Here, we demonstrate the determination of the crystal structures of T. brucei GMPR; a protein that, unlike the GMPRs of host animals, possesses a CBS domain. We further show that TbGMPR activity is regulated by purine nucleotide binding to an allosteric regulatory site formed at the cleft between the catalytic and CBS domains of the enzyme. Our kinetic and structural analyses clearly demonstrate that the CBS domain has a pivotal role in the allosteric regulation of the activity and structure of TbGMPR, facilitating the transitions among three conformations: a tetramer, and octamers with relaxed and twisted conformations. A combination of X-ray crystallography and size-exclusion chromatography small-angle X-ray scattering (SEC-SAXS) analysis clearly revealed that TbGMPR can exist as a tetramer or an octamer depending on the nucleotide species that is bound to the CBS domain.

We also determined the structure of TbGMPR C318A with substrate GMP (C318A/GMP) at 1.90-Å resolution and found that C318A/GMP adopted an octameric structure as observed in C318A apo. However, two tetramers in the C318A/GMP octamer were arranged in a twisted position around the fourfold axis compared to C318A apo, and the overall structure of the C318A/GMP octamer was compressed along the fourfold axis. Thus, it appears that GMP induces the transformation of TbGMPR from a “relaxed” (C318A apo) to a “twisted” form (C318A/GMP). Two GMP molecules were observed in each subunit of C318A/GMP; one was found in the active site, whereas the other was bound to the cleft between the catalytic and CBS domains. The interactions between the active site and the substrate GMP molecule involved 12 hydrogen bonds and 7 C–C contacts. The interactions between the base moiety of GMP and three amino acid residues (Met401, Ala402, and Glu428) in the catalytic domain appeared to stabilize the α-helix and a portion of the following loop structure that were disordered in C318A apo. The ligand GMP molecule at the allosteric regulatory site formed 10 hydrogen bonds to and exhibited 13 hydrophobic interactions with the amino acid residues in the CBS domain; at the same time, the O6 and N7 atoms in the GMP molecule interacted with Arg93 in the catalytic domain via hydrogen bonds. The structures of the isolated catalytic and CBS domains in C318A/GMP could be well-superposed with the respective domains in C318A apo. However, the relative orientation of these domains was obviously different between C318A/GMP and C318A apo: the CBS domain is rotated ~40° between these two structures, a change that may be induced by an interaction between the base moiety of GMP and Arg93. This hinge motion is inferred to contribute to the transformation from the relaxed to the twisted octamer.

> MSFNESASIPTGLTYDDVLIIPQHSRVTSRKEVNTTTRLSRNVKLSIPIVASNMDTVCEQRMAVAMAREGGIGILHRFCSIEEQCAMLREVKRAQSFLIESPRIILPHETAREAWEGLNWKGRVGGVGCLLVVNCKNERKLLGIITRHDLKLADESTTVESLMTPVDKMVVSTNTSISLEEVTHLMRKGRTANVPIVGQNGQLLYLVTLSDVVKLRKNKQASLDSRGRLLVGAAVGVKKDDMNRAIRLVEAGADVLVVDIAHGHSDLCINMVKRLKGDPRTASVDIIAGNIASAEAAEALIDAGADGLKIGVGPGSIAITRLVAGAGVPQLSAVLACTRVARRRGVPCIADGGLRTSGDISKAIGAGADTVMLGNMLAGTDEAPGRVLVKDGQKVKIIRGMAGFGANLSKAERERTQDEDVFSSLVPEGVEGSVACKGPVGPIVRQLVGGLRSGMSYSGAKSIEEMQRRTRFVRMTGAGLRESGSHGVAKLKLAAALEHHHHHH> QAKHKQRKRLKSSCKRHPLYVDFSDVGWNDWIVAPPGYHAFYCHGECPFPLADHLNSTNHAIVQTLVNSVNSKIPKACCVPTELSAISMLYLDENEKVVLKNYQDMVVEGCGCR;> ETGQCRIQKCTTDFVSLTSHLNSAVDGFDSEFCKALRAYAGCTQRTSKACRGNLVYHSAVLGISDLMSQRNCSKDGP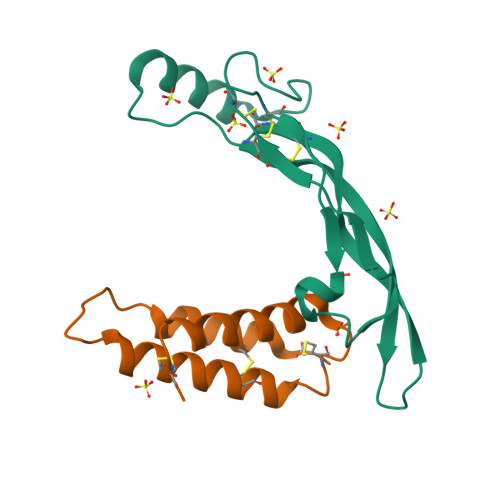TSSTNPEVTHGTKHHHHHH> NELEEMQRRADQLADESLESTRRMLQLVE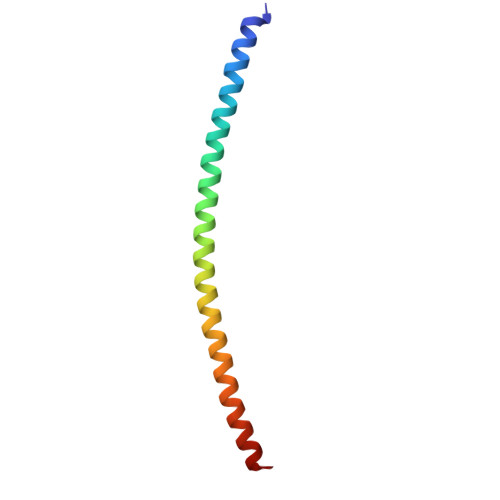ESKDAGIRTLVMLDEQGEQLDRVEEGMNHINQDMKEAEKNLKDLGK>[4x]MPMILGYWDIRGLAHAIRLLLEYTGSDYEEKIYSMGDAPDYDRSQWLSEKFKLGLDFPNLPYLIDGAHRLTQSNAILRYIARKHNLCGETE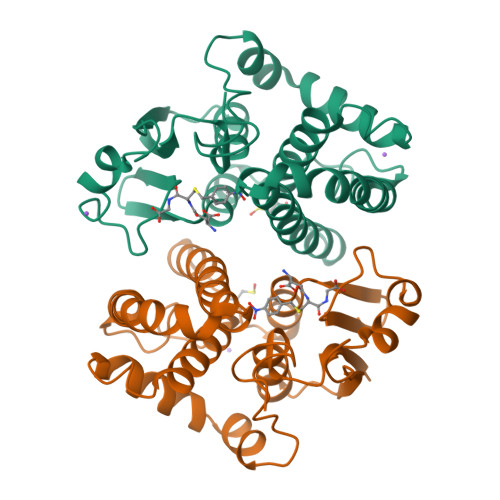EEKIRVDVLENQAMDTRLDFARVCYNPDFEKLKPGFLKEIPEKMKLFSEFLGKRTWFAGDKLNYVDFLAYDVLDVYRIFEPKCLDEFPNLKDFMSRFEGLKKISAYMKSSRFLRSPLFLKMAMWGNK(2R,3Z)-3-amino-3-imino-2-[(E)-phenyldiazenyl]propanamide | C9 H11 N5 O | 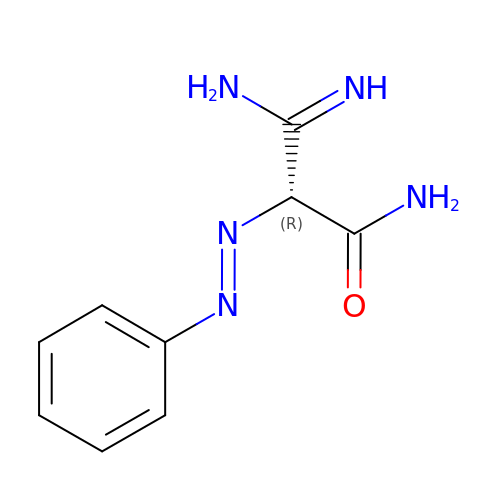IWQCRGGEGLIWHV-KJZWZZJGSA-N>[2x]MFEQRVNSDVLTVSTVNSQDQVTQKPLRDSVKQAL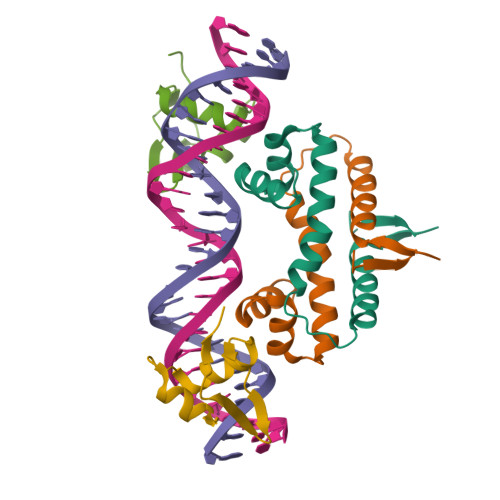KNYFAQLNGQDVNDLYELVLAEVEQPLLDMVMQYTRGNQTRAALMMGINRGTLRKKLKKYGMN;>MYLTLQEWNARQRRPRSLETVRRWVRESRIFPPPVKDGREYLFHESAVKVDLNRP[2x]>MVQPFAWQVASLADRYEESFDIGAAVEPHQLNGRQGKVLKHHYNSIVAENAMKPISLQPEEGVFTWDGADAIVEFARKNNMNLRFHTLVWHNQVPDWFFLDEEGNPMVEETNEAKRQANKELLLERLETHIKTVVERYKDDVTAWDVVNEVVDDGTPNERGLRESVWYQITGDEYIRVAFETARKYAGEDAKLFINDYNTEVTPKRDHLYNLVQDLLADGVPIDGVGHQAHIQIDWPTIDEIRTSMEMFAGLGLDNQVTELDVSLYGWPPRPAFPTYDAIPQERFQAQADRYNQLFELYEELDADLSSVTFWGIADNHTWLDDRARE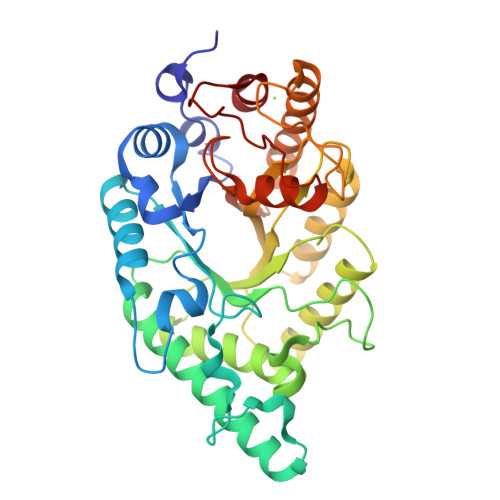YNDGVGKDAPFVFDPNYRVKPAFWRIID[2x]>[3x]MRTTKFLALALCLLASASALSANNSAPSNDWWDIPYPSQFDVKSLKTQSFISVKGNKFIDDKGKTFTFRGVNIADTGKLLSRNQWQKSLFEELANNWGVNTIRLPIHPVSWRKLGPDVYLGHIDEAVRWANDLGIYLILDWHSIGYLPTEQYQHPMYDTTIKETRDFWRRITFRYQNVPTVA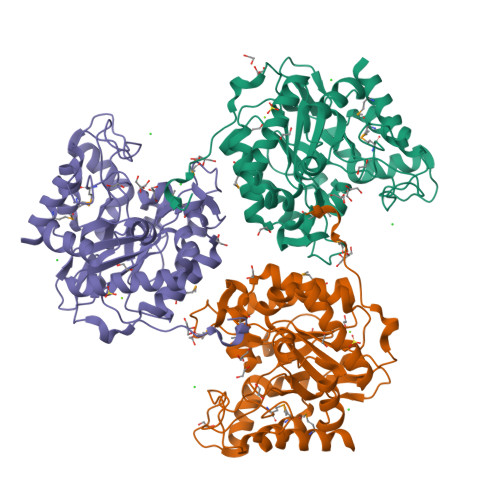VYELFNEPTTMGNTLGERNWAEWKTLNESLIDMIYASDKTVIPLVAGFNWAYDLSPIKKAPIEREGIAYAAHPYPQKAKPEVKNDKNFFKLWDEKWGFAADTYPVIATELGWVQPDGYGAHIPVKDDGSYGPRIVKYMQKKGVSYTVWVFDPDWSPTMINDWDFTPSEQGAFFKQVMLEAKKR>GPGSMVAGQAGSLQGRVAFITGAARGQGRSHAVRLAAEGADIIACDICAPVSASVTYAPASPEDLDETARLVEDQGRKALTRVLDVRDDAALRELVADGMEQFGRLDVVVANAGVLSWGRVWELTDEQWDTVIGVNLTGTWRTLRATVPAMIEAGNGGSIVVVSSSAGLKATPGNGHYSASKHGLTALTNTLAIELGEYGIRVNSIHPYSVETPMIEPEAMMEIFARHPSFVHSFPPMPVQPNGFMTADEVADVVAWLAGDGSGTLTGTQIPVDKGALKY[4x]

Here we present a series of TIGR03971 SDR crystal structures from several mycobacterial species which contain an insertion in the primary sequence at the NAD cofactor binding site. These crystal structures demonstrate that the inserted protein residues almost completely cover the NAD cofactor, only leaving part of the nicotinamide ring exposed to solvent. NMR experiments did not show exchange of the NAD cofactor, whereas binding was demonstrated for a number of small molecules which could be potential substrates, products, inhibitors, or artificial redox partners. Experimental results are consistent with the notion that the SDR family enzymes linked by comparative genomics studies to mycofactocin do indeed keep their NAD tightly bound beneath a protein structure that may interact with a specialized adaptor machinery for redox exchange.

With the exception of the M. thermoresistibile target which did not contain NAD, all other mycobacterial SDR target crystal structures contained NAD, which appears to have co-purified with the protein after expression in E. coli. For each of these crystal structures, the adenosine mononucleotide portion of the cofactor binding site is enveloped by the inserted residues and only a portion of the nicotinamide ring appears open to solvent (see representative examples in Fig. 2A and B). In addition to the insertion loop which covers the adenosine portion of the cofactor, a second loop which typically contains two α-helices covers much of nicotinamide mononucleotide portion of the cofactor. In contrast, this loop is ordered in each of the mycobacterial SDR crystal structures presented here. The combination of the insertion loop which covers the adenosine portion of the cofactor and the ordering of the second loop which covers the nicotinamide mononucleotide portion of the cofactor results in a significant decrease in the solvent accessible surface area of the cofactor in the mycobacterial SDRs, relative to other NAD- and NADP-dependent dehydrogenases. Only a small portion of the nicotinamide ring appears available to solvent in each of these cases, indicating that the NAD cofactor is tightly bound and potentially non-exchangeable. The structures presented here have a cofactor solvent accessible surface area of approximately 18 Å2, whereas other NAD- or NADP-bound dehydrogenases have a cofactor solvent accessible surface area of 82–89 Å2. Given the encapsulation of the NAD cofactor by the two loops in mycobacterial SDRs, a large conformational change would be required to release the NADH cofactor after a redox reaction had occurred. Alternatively, these structural elements may not allow for exchange of bound NAD/NADH with free NAD/NADH.>MAAACRSVKGLVAVITGGASGLGLATAERLVGQGASAVLLDLPNSGGEAQAKKLGNNCVFAPADVTSEKDVQTALALAKGKFGRVDVAVNCAGIAVASKTYNLKKGQTHTLEDFQRVLDVNLMGTFNVIRLVAGEMGQNEPDQGGQRGVIINTASVAAFEGQVGQAAYSASKGGIVGMTLPIARDLAPIGIRVMTIAPGLFGTPLLTSLPEKVCNFLASQVPFPSRLGDPAEYAHLVQAIIENPFLNGEVIRLDGAIRMQP[4x];> SRPRKDPLRHLRTREKRGPSGCSGGPNTVYLQVVAAGSRDSGAALYVFSEFNRYLFNCGEGVQRLMQEHKLKVARLDNIFLTRMHWSNVGGLSGMILTLKETGLPKCVLSGPPQLEKYLEAIKIFSGPLKGIELAVRPHSAPEYEDETMTVYQIPIHSEQRRGKHQPWQSPERPLSRLSPERSSDSESNENEPHLPHGVSQRRGVRDSSLVVAFICKLHLKRGNFLVLKAKEMGLPVGTAAIAPIIAAVKDGKSITHEGREILAEELCTPPDPGAAFVVVECPDESFIQPICENATFQRYQGKADAPVALVVHMAPASVLVDSRYQQWMERFGPDTQHLVLNENCASVHNLRSHKIQTQLNLIHPDIFPLLTSFRCKKEGPTLSVPMVQGECLLKYQLRPRREWQRDAIITCNPEEFIVEALQLPNFQQSVQEYRRSAQDGPAPAEKRSQYPEIIFLGTGSAIPMKIRNVSATLVNISPDTSLLLDCGEGTFGQLCRHYGDQVDRVLGTLAAVFVSHLHADHHTGLPSILLQRERALASLGKPLHPLLVVAPNQLKAWLQQYHNQCQEVLHHISMIPAKCLQEGAEISSPAVERLISSLLRTCDLEEFQTCLVRHCKHAFGCALVHTSGWKVVYSGDTMPCEALVRMGKDATLLIHEATLEDGLEEEAVEKTHSTTSQAISVGMRMNAEFIMLNHFSQRYAKVPLFSPNFSEKVGVAFDHMKVCFGDFPTMPKLIPPLKALFAGDIEEMEERREKRELRQVRAALLSRELAGGLEDGEPQQKRAHTEEPQAKKVRAQ;> MKSSVQEECVSTISSSKDEDPLAATREFIEMWRLLGREVPEHITEEELKTLMECVSNTAKKKYLKYLYTKEKVKKARQIKKEMKAAAREEAKNIKLLETTEEDKQKNFLFLRLWDRNMDIAMGWKGAQAMQFGQPLVFDMAYENYMKRKELQNTVSQLLESEGWNRRNVDPFHIYFCNLKIDGALHRELVKRYQEKWDKLLLTSTEKSHVDLFPKDSIIYLTADSPNVMTTFRHDKVYVIGSFVDKSMQPGTSLAKAKRLNLATECLPLDKYLQWEIGNKNLTLDQMIRILLCLKNNGNWQEALQFVPKRKHTGFLEISQHSQEFINRLKKAKTAENLYFQSHHHHHHDYKDDDDK

Here, we present several cryo-EM structures of the mitochondrial RNase Z complex (ELAC2/SDR5C1/TRMT10C) bound to different maturation states of mitochondrial tRNAHis, showing the molecular basis for tRNA-substrate selection and catalysis. The human long form of RNase Z, ELAC2, has two alternative start codons to produce a nuclear and a mitochondrially targeted form. TRMT10C is a purine N1-methyltransferase that acts at position 9 of mt-tRNAs using S-adenosylmethionine (SAM) as a co-substrate. SDR5C1 is a moonlighting homotetrameric short-chain dehydrogenase/reductase.

The TRMT10C/SDR5C1 platform in the RNase Z-HCCA complex is similar to the RNase Z-HS and RNase ZH548A-HS complexes, but here, ELAC2 pivots by ~6 degrees around the tRNA (Fig. EV3A). Consequently, the active site is now ~13 Å away from the mt-tRNAHis 3′-end, and the active site channel is occupied by the 3′-CCA tail. The first C (C1CCA) of the 3′-CCA tail is recognized by H-bonding to S726 and S490 and to the backbone carbonyls 490 and 492, which lie at the entrance of the active site channel. The second C (C2CCA) inserts into a pocket in the NTD situated on the opposite side of the active site channel. C2CCA establishes H-bonds with Q92 and T127, which pulls C2CCA toward the bottom of the pocket. Furthermore, the phosphodiester bond between C1CCA and C2CCA is stabilized by K700. The C1CCA–C2CCA bond is the closest to the active site. Nevertheless, it is not well positioned for hydrolysis since it is 1.9 Å further away from the active site than the scissile bond in the mt-tRNAHis-Ser(AGY) complex. Furthermore, the phosphate oxygens point away from the active site Zn2+, so they cannot participate in the hydrolysis reaction catalyzed by ELAC2.>MAEQRQLHLAGFFSAGNVTHAHGAWRHVGATNGFLTGEFYKQIARTLERGKFDLLFLPDGLAIEDSYGDNLETGVGLGGQGAVALEPTSVIATMAAVTQRLGLGATVSTTYYPPYHVARVFATLDNLSDGRISWNVVTSLNDSEARNFGVDEHLEHDIRYDRADEFLEAVKKLWSSWSEDALLLDKVGGRFADPKKVQYVNHRGRWLSVRGPLQVPRSRQGEPVILQAGLSPRGRRFAGRWAEAVFSVSPNLDIMRAVYQDIKAHVAAAGRDPEQTKVFTAVMPVLGETEQVARERLEYLNSLVHPEVGLSTLSSHSG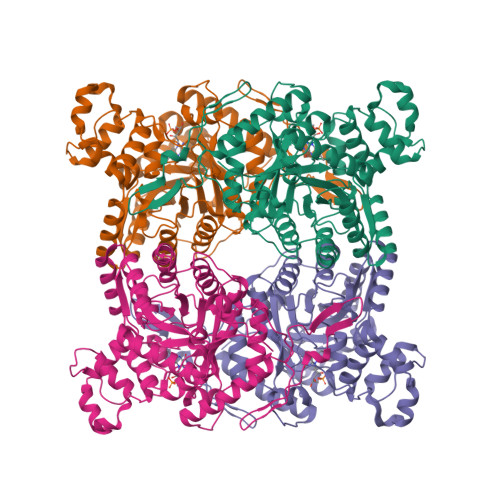LNLSKYPLDTKFSDIVADLGDRHVPTMLQMFSAVAGGGADLTLAELGRRYGTNVGFVPQWAGTAEQIADQLISHFEAGAADGFIISPAYLPGIYEEFVDQVVPLLQQRGVFRTEYEGTTLREHLGLAHPEVGSIR[4x]>[4x]GKLSEHLRYCDSILREMLSKKHAAYAWPFYKPVDAEALEL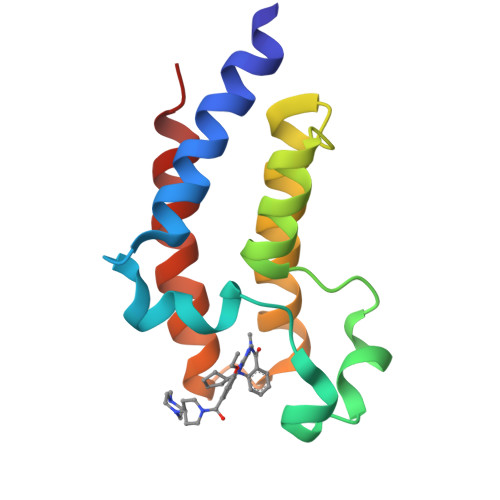HDYHDIIKHPMDLSTVKRKMDGREYPDAQGFAADVRLMFSNCYKYNPPDHEVVAMARKLQDVFEMRFAKMP>[2x]RPSSRVYIVEVLNEFPHDPYAFTQGLVYAENDTLFESTGLYGRSSVRQVALQTGKVENIHKMDDSYFGEGLTLLNEKLYQVVWLKNIGF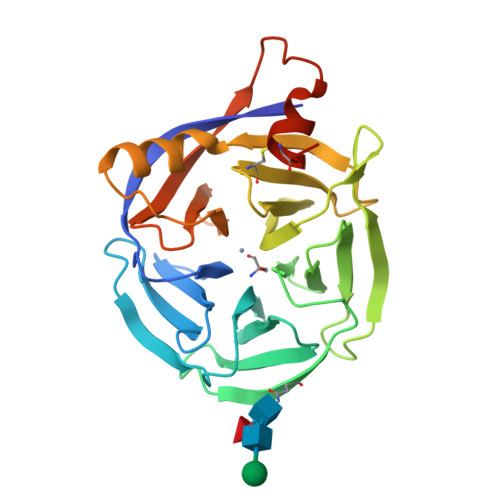IYDRRTLSNIKNFTHQMKDGWGLATDGKILYGSDGTSILYEIDPHTFKLIKKHNVKYNGHRVIRLNELEYINGEVWANIWQTDCIARISAKDGTLLGWILLPNLRKKLIDEGFRDIDVLNGIAWDQENKRIFVTGKLWPKLFEIKLHLVRHRIPDGYIERHCLNLRDNTLSLKTDID> HMHGRLKVKTSEEQAEAKRLEREQKLKLYQSATQAVFQKRQAGELDESVLELTSQILGANPDFATLWNCRREVLQHLE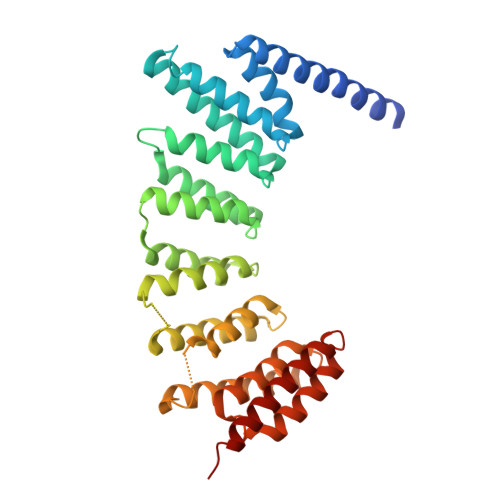TEKSPEESAALVKAELGFLESCLRVNPKSYGTWHHRCWLLSRLPEPNWARELELCARFLEADERNFHCWDYRRFVAAQAAVAPAEELAFTDSLITRNFSNYSSWHYRSCLLPQLHPQPDSGPQGRLPENVLLKELELVQNAFFTDPNDQSAWFYHRWLLGAGSGRCELSVEKSTVLQSELESCKELQELEPENKWCLLTIILLMRALDPLLYEKETLQYFSTLKAVDPMRAAYLDDLRSKFLLENSVLKMEYA>MALQEIEFTSHNGRDAIQAWAYEPVGTPTAVVQIIHGLGEHSRRYLHMISALLDAGFVVIADDHAGHGRTAMQSGVWADAGDNAAEVVISDELTLQQQLAGQFDDLPWVVFGHSWGSMIARAMATRPGTRLDGLALCGIVAQPRGFETTLDHKTLAKAMATAPTDPAPEALVAQMFDGFADRLSEDDGPTGWVARSKEVVADHGKDKFNNFGAPMSTRFLQGLADIYAMANGDSFYATMPNIPIVLFAGSEDPAGDFGTGVKAVAERLRRDGHNVELHLYDG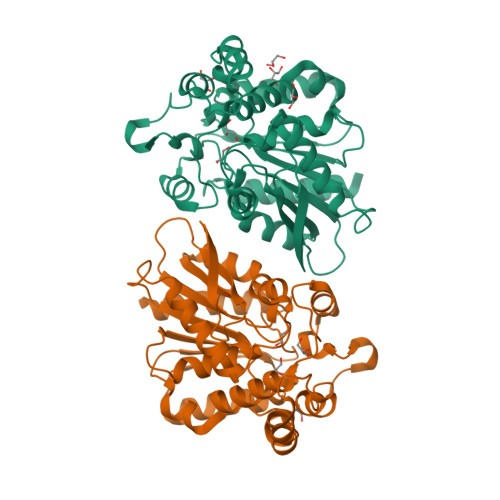LRHEVHNEPESRADVESSLVTFVDRVANRRIKRSR[2x]>[2x]GKPLHEQLWYHGAIPRAEVAELLVHSG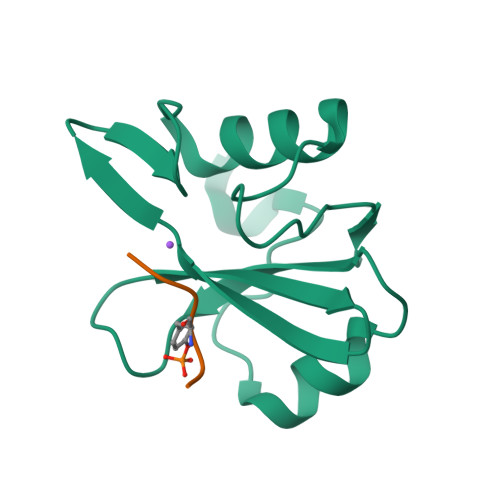DFLVRESETVKGAYALSVLWDGLPRHFLIQSLDNLYRLEGEGFPSIPLLIDHLLSTQQPLTKKSGVVLHRAVP;>PPVYEPV[2x]> VHITLDPDTANPWLILSEDRRQVRLGDTQ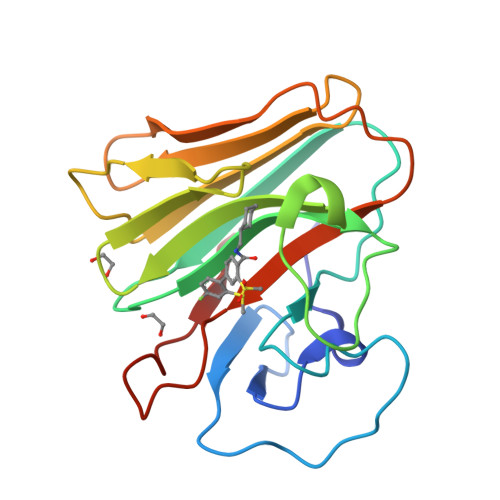QSIPGNEERFDSYPMVLGAQHFHSGKHYWEVDVTGKEAWDLGVCRDSVRRKGHFLLSSKSGFWTIWLWNKQKYEAGTYPQTPLHLQVPPCQVGIFLDYEAGMVSFYNITDHGSLIYSFSECAFTGPLRPFFSPGFNDGGKNTAPLTLCPL> EDLLKNLLTMGVDIDMARKRQPGVFHRMITNEQDLKMFLLSKGASKEVIASIISRYPRAITRTPENLSKRWDLWRKIVTSDLEIVNILERSPESFFRSNNNLNLENNIKFLYSVGLTRKCLCRLLTN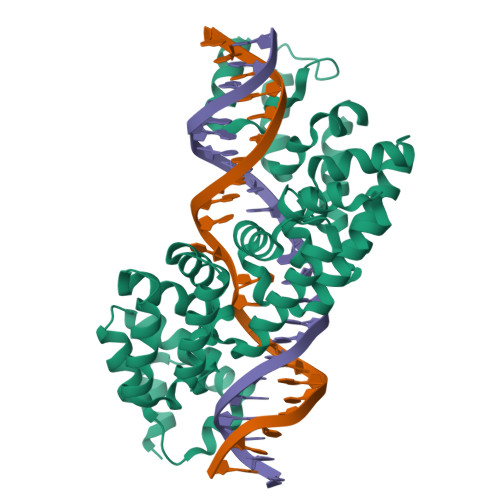APRTFSNSLDLNKQMVEFLQAAGLSLGHNDPADFVRKIIFKNPAILIQSTKRVKANIEFLRSTFNLNSEELLVLICGPGAEILDLSNDYARRSYANIKEKLFSLGCTEEEVQKFVLSYPDVIFLAEKKFNDKIDCLMEENISISQIIENPRVLDSSISTLKSRIKELVNAGCNLSTLNITLLSWSKKRYEAKLKKLS GLYCINAMIDE 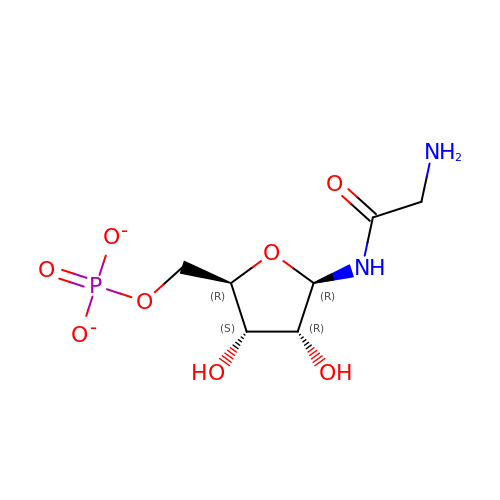RIBONUCLEOTIDE | C7 H13 N2 O8 P | OBQMLSFOUZUIOB-SHUUEZRQSA-L> GSHMSDKPLTKTDYLMRLRRCQTIDTLERVIEKNKYELSDNELAVFYSAADHRLAELTMNKL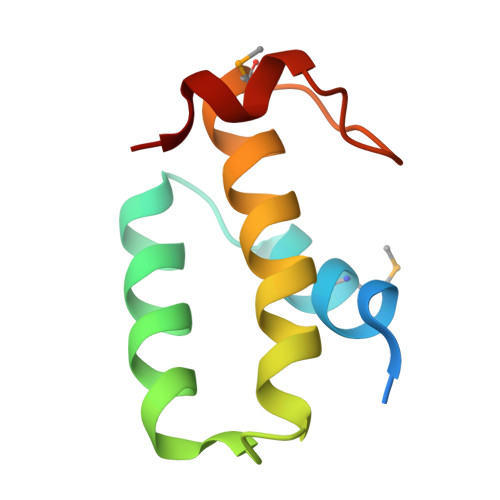YDKIPSSVWKFIR N-[(5R,14R)-5-AMINO-5,14-DIMETHYL-4-OXO-3-OXA-18-AZATRICYCLO[15.3.1.1~7,11~]DOCOSA-1(21),7(22),8,10,17,19-HEXAEN-19-YL]-N-METHYLMETHANESULFONAMIDE | C24 H33 N3 O4 S | 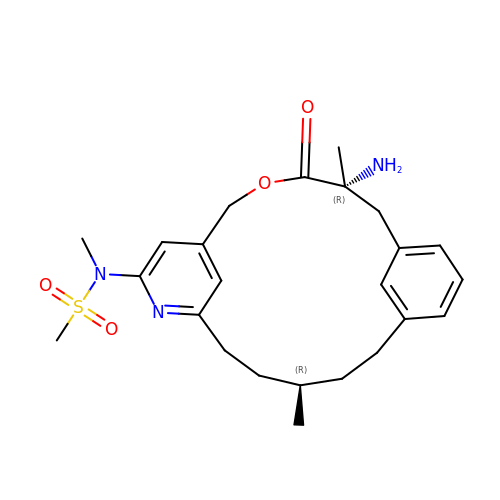QWDOKZPZLWNULU-MZNJEOGPSA-N>[32x]MGKHHHHHHGSLEVLFQGPMSSRSTGSFDEISQYIQELEEERR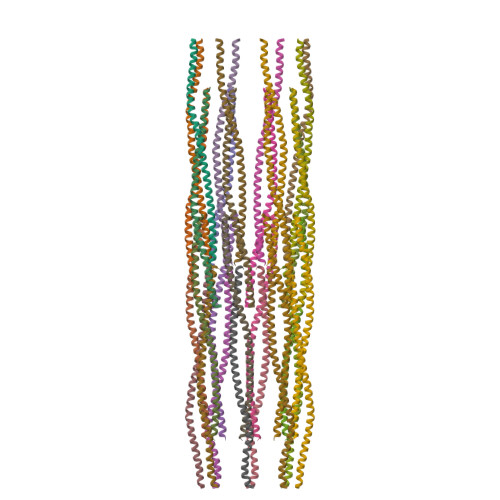LTESSIRKMEKEKSDLNEKIDELTTRKCSVDARLQAENERAERQDRGLKEAETTYAKLVESQKTLVDFVRKEYEDTKHQKY> SNAMQNRWAETKFDSDIDEVVYGSRLIGSDPDLVLHGGGNTSVKTTERDHAGRIISVLRVKNSGSNLGTIDSRGFTGIRMDDALAAAKIDKMTDEAMVDYLKKSMVNPSEPSPSVETFLHAFLPYKFVMHSHADAILSITNTDLPSDQIAKILGNVVVLPYIPPGFTLAKEVMNCFKKGIDGIVLRKHGLLTFGDTGKEAYD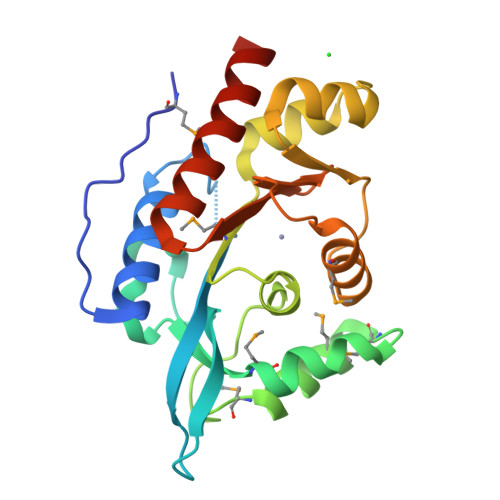RHINIVSRAENFIREKTDGK In platelets, scrambling is mediated by the protein TMEM16F, which catalyzes the externalization of phosphatidylserine (PS) in response to an increase in the intracellular Ca2+ concentration to trigger blood clotting. TMEM16F belongs to the TMEM16 protein family, whose members either function as Ca2+ activated anion-selective channels or as Ca2+ activated lipid scramblases. To better understand how the small sequence differences in TMEM16F give rise to its distinct functional properties, we determined the structure of murine TMEM16F (mTMEM16F) by cryo-EM in Ca2+-bound and Ca2+-free states, both in a detergent and in a lipid environment. By combining data from cryo-electron microscopy, in vitro scrambling assays and electrophysiology, our study has provided insight into the diverse functional behavior of mTMEM16F, a member of the TMEM16 family that facilitates the transport of lipids and ions across cellular membranes. Both processes are controlled by the binding of Ca2+ to a site located within the transmembrane domain that is accessible from the cytoplasm and they are mediated by the same structural element located at the periphery of each subunit.

For that purpose, we determined structures of mTMEM16F in the absence and presence of Ca2+. Structures of the protein in the detergent digitonin were determined for Ca2+-bound and Ca2+-free states by cryo-EM at 3.2 Å and 3.6 Å, respectively (Figure 2—figure supplements 1 and 2). The structure of mTMEM16F in the presence of Ca2+ defines the location of two Ca2+ ions in each subunit that are bound to a site which strongly resembles its counterpart in nhTMEM16 and mTMEM16A. In this site, conserved acidic and polar residues located on α-helices 6–8 coordinate the ions with similar geometry. In the presence of Ca2+, the bound ligands provide an interaction platform for negatively charged and polar residues on α6, thereby immobilizing the helix in the observed conformation. The structure of the putative catalytic unit of mTMEM16F in a Ca2+-bound conformation shows a strong resemblance to the ion permeation path in mTMEM16A, where an hourglass-shaped pore contains two aqueous vestibules on either side of the membrane that are bridged by a narrow neck. A related architecture is observed in mTMEM16F, where closer interactions between α-helices and the presence of bulky residues along the path further constrict the pore below the size of permeating ions. Further towards the cytoplasm, the bulky Tyr 563 lowers the pore diameter of mTMEM16F to 1.6 Å. In the case of Ca2+-bound structures, the relationship of mTMEM16F to the intermediate conformation of nhTMEM16 observed in nanodiscs is, with an RMSD of 1.9 Å, much closer than to the open conformation of the same protein, where the RMSD of 3.1 Å underlines their nonequivalence.

>MQMMTRKVLLNMELEEDDDEDGDIVLENFDQTIVCPTFGSLENQQDFRTPEFEEFNGKPDSLFFTDGQRRIDFILVYEDESKKENNKKGTNEKQKRKRQAYESNLICHGLQLEATRSVSDDKLVFVKVHAPWEVLCTYAEIMHIKLPLKPNDLKTRSPFGNLNWFTKVLRVNESVIKPEQEFFTAPFEKSRMNDFYILDRDSFFNPATRSRIVYFILSRVKYQVMNNVNKFGINRLVSSGIYKAAFPLHDCRFNYESEDISCPSERYLLYREWAHPRSIYKKQPLDLIRKYYGEKIGIYFAWLGYYTQMLLLAAVVGVACFLYGYLDQDNCTWSKEVCDPDIGGQILMCPQCDRLCPFWRLNITCESSKKLCIFDSFGTLIFAVFMGVWVTLFLEFWKRRQAELEYEWDTVELQQEEQARPEYEAQCNHVVINEITQEEERIPFTTCGKCIRVTLCASAVFFWILLIIASVIGIIVYRLSVFIVFSTTLPKNPNGTDPIQKYLTPQMATSITASIISFIIIMILNTIYEKVAIMITNFELPRTQTDYENSLTMKMFLFQFVNYYSSCFYIAFFKGKFVGYPGDPVYLLGKYRSEECDPGGCLLELTTQLTIIMGGKAIWNNIQEVLLPWVMNLIGRYKRVSGSEKITPRWEQDYHLQPMGKLGLFYEYLEMIIQFGFVTLFVASFPLAPLLALVNNILEIRVDAWKLTTQFRRMVPEKAQDIGAWQPIMQGIAILAVVTNAMIIAFTSDMIPRLVYYWSFSIPPYGDHTYYTMDGYINNTLSVFNITDFKNTDKENPYIGLGNYTLCRYRDFRNPPGHPQEYKHNIYYWHVIAAKLAFIIVMEHIIYSVKFFISYAIPDVSKITKSKIKREKYLTQKLLHESHLKDLTKNMGIIAERIGGTVDNSVRPKLE[2x]>[2x]MSGAPPGYRPSAWVHLLHQLPRADFQLRPVPSVFAPQEQEYQQALLLVAALAGLGLGLSLIFIAVYLIRFCCCRPPEPPGSKIPSPGGGCVTWSCIVALLAGCTGIGIGFYGNSETSDGVSQLSSALLHANHTLSTIDHLVLETVERLGEAVRTELTTLEEVLEPRTELVAAARGARRQAEAAAQQLQGLAFWQGVPLSPLQVAENVSFVEEYRWLAYVLLLLLELLVCLFTL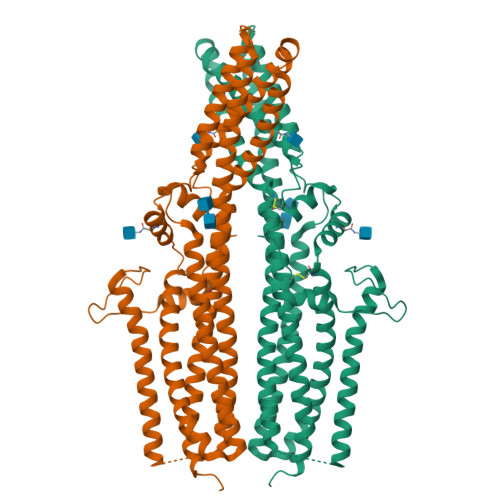LGLAKQSKWLVIVMTVMSLLVLVLSWGSMGLEAATAVGLSDFCSNPDPYVLNLTQEETGLSSDILSYYLLCNRAVSNPFQQRLTLSQRALANIHSQLLGLEREAVPQFPSAQKPLLSLEETLNVTEGNFHQLVALLHCRSLHKDYGAALRGLCEDALEGLLFLLLFSLLSAGALATALCSLPRAWALFPPSDDYDDTDDDDPFNPQESKRFVQWQSSIALEVLFQ ethyl 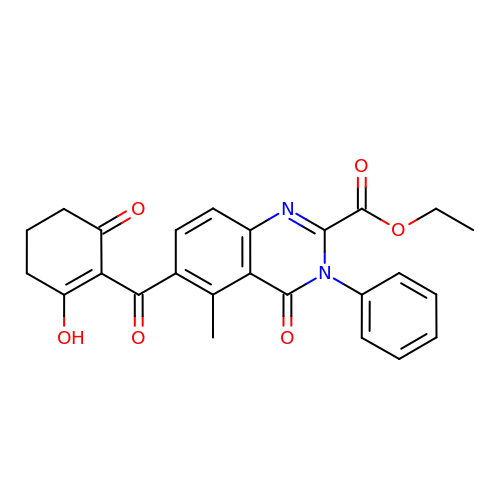5-methyl-4-oxidanylidene-6-(2-oxidanyl-6-oxidanylidene-cyclohexen-1-yl)carbonyl-3-phenyl-quinazoline-2-carboxylate | C25 H22 N2 O6 | AUUQMCPECJKYRI-UHFFFAOYSA-N> NGDRLYKADSRPPDEIKRSGGLMPRGHNEYFDRGTQMNINLYDHARGTQTGFVRYDDGYVSTSLSLRSAHLAGQSILSGYSTYYIYVIATAPNMFNVNDVLGVYSPHPYEQEVSALGGIPYSQIYGWYRVNFGVIDERLHRNREYRDRYYRNLNIAPAEDGYRLAGFPPDHQAWREEPWIHHAPQGCGNSS;> RTITGDTCNEETQNLSTIYLREYQSKVKRQIFSDYQSEVDIYNRIRDEL;>APQTITELCSEYRNTQIYTINDKILSYTESMAGKREMVIITFKSGETFQVEVPGSQHIDSQKKAIERMKDTLRIT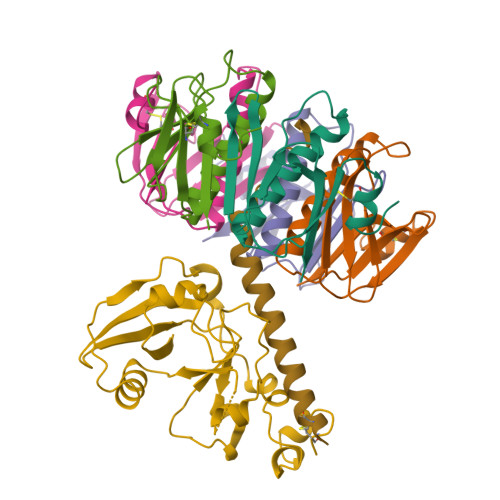YLTETKIDKLCVWNNKTPNSIAAISMKN[5x]DICHLORO-ACETIC ACID | C2 H2 Cl2 O2 | 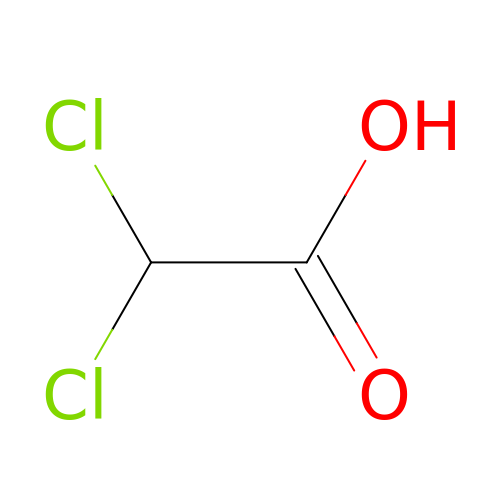JXTHNDFMNIQAHM-UHFFFAOYSA-N(S)-IBUPROFENOYL-COENZYME A | C34 H53 N7 O17 P3 S | 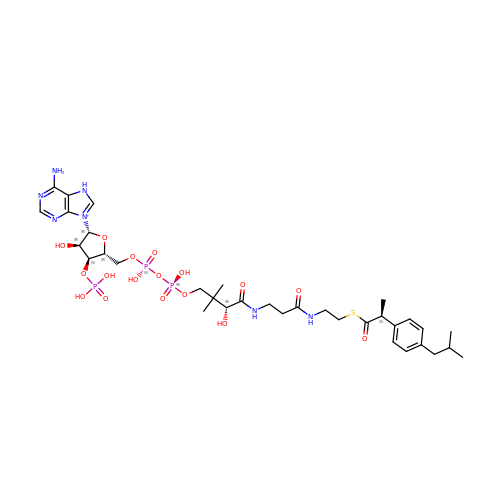NXIKDQUQQHUCJH-MIXAKNBRSA-O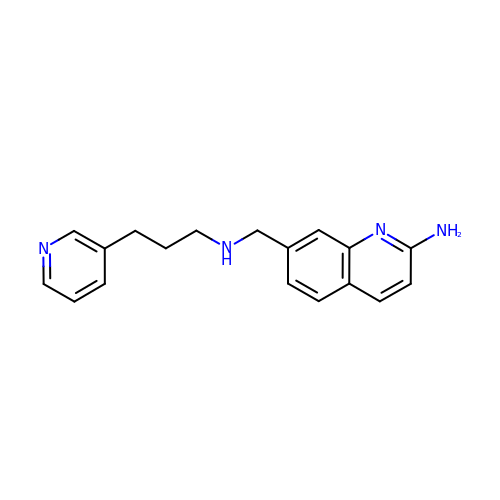7-(((3-(PYRIDIN-3-YL)PROPYL)AMINO)METHYL)QUINOLIN-2- | C18 H20 N4 | SYLCHGGIDVOGEK-UHFFFAOYSA-N> MKSRTSELAVGIFVIIFGIALFFLAMKVSGLVGTNLSDGYTMKAQFDNVNGLKPRAKVTMSGVTIGRVDS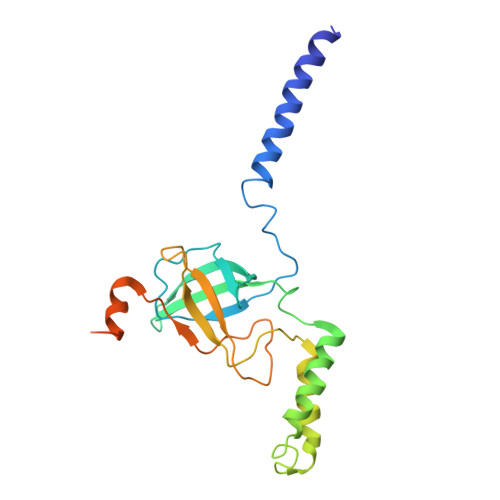ITLDPVTRLATVTFDLDGKLTSFNAEQLKEVQKNALDELRYSSDYTQATPAQQKTMEQQLISNMNSITSIDEDAYIMVATNGLLGEKYLKIVPGGGLNYLKRGDTISNTQGTMDLEDLISKFITGGGAGKVAAGSSSAEEKAPASTDSSAQP>MPNIKIFSGSSHQDLSQKIADRLGLELGKVVTKKFSNQETCVTIGESVRGEDVYIVQSGCGEINDNLMELLIMINACKIASASRVTAVIPCFPYARQDKKDKSRAPISAKLVANMLSVAGADHIITMD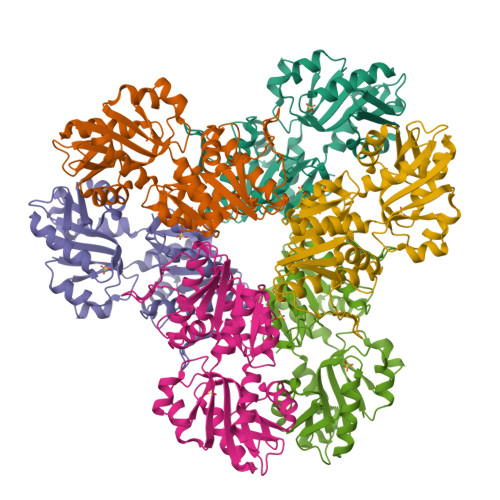LHASQIQGFFDIPVDNLYAEPAVLKWIRENISEWRNCTIVSPDAGGAKRVTSIADRLNVDFALIHKERKKANEVDRMVLVGDVKDRVAILVDDMADTCGTICHAADKLLSAGATRVYAILTHGIFSGPAISRINNACFEAVVVTNTIPQEDKMKHCSKIQVIDISMILAEAIRRTHNGESVSYLFSHVPLLEHHHHHH[2x]The methylsuccinyl-CoA dehydrogenase (MCD)3 is a member of the flavin-dependent acyl-CoA dehydrogenase (ACD) family. MCD catalyzes the oxidation of the α-branched (2S)-methylsuccinyl-CoA into the corresponding trans-2-enoyl-CoA thioester, mesaconyl-CoA. The enzyme plays a crucial role in the ethylmalonyl-CoA pathway for acetyl-CoA assimilation in many α-proteobacteria (e.g. Rhodobacter sphaeroides, Methylobacterium extorquens, and Paracoccus denitrificans), actinobacteria (e.g. Streptomyces spp. and Frankia spp.), and possibly spirochaetes (e.g. Leptospira spp.). The α,β-desaturation of the CoA thioester is initiated by a proton abstraction from the α-carbon by a conserved catalytically active glutamate and a hydride transfer from the β-carbon to the N5 of the FAD cofactor.

Here we report the high resolution structure of MCD from P. denitrificans (PdMCD) that catalyzes the unprecedented α,β-desaturation of an α-methyl branched dicarboxylic acid CoA thioester. PdMCD forms a homodimer, consistent with our gel filtration analysis. The obtained well-ordered high-resolution electron density map allowed us to model almost the entire polypeptide chain (missing only 10 N-terminal residues) as well as the FAD cofactor in both active sites. Nevertheless, we also observed electron densities at the surfaces of each monomer that allowed the modeling of the adenosyl phosphate parts of CoA or its derivative. In contrast to canonical tetrameric ACDs, PdMCD possesses an additional ∼170-amino acid extension at the N terminus. However, when superimposing the PdMCD monomer with the MCAD tetramer, it becomes apparent that the N-terminal ∼170-residue extension of PdMCD structurally mimics the dimer–dimer interface of MCAD. By emulating the dimer–dimer interface found in the tetrameric ACDs, the N-terminal extension of PdMCD probably stabilizes the PdMCD dimer. The cofactor FAD binds to PdMCD in a “drawn-out” conformation, as observed for other ACDs. Both subunits of the MCD dimer contribute to the binding of FAD, which adopts a “butterfly-like” conformation in respect to the isoalloxazine ring. In PdMCD, however, helix E is shifted >2 Å to the back of the active site compared with IBD and MCAD, providing even more space, probably to accommodate the terminal carboxylic acid group of methylsuccinyl-CoA. The carboxylic acid group of the substrate could potentially interact with three arginine residues (Arg-252, Arg-376, and Arg-421) that are all in close proximity.

>MKDMPAMPADTPSALLALAGEALPELESLQSRATEALRALVAPAGKPQPALLEQHQHAAHALSWLTTYVESIRQLSGWAGRLAEAGNLGRIEALILQIGLGEYLGQIAGGIPMSQTEFARLSDLELDWQPGEAAAKLMRGNTAPARAELARLMQDNHGRATFGATGLDEDLEMIRDQFRRYAEERVIPNAHEWHLKDQLIPMEIIEELAELGVFGLTIPEEFGGLGLSKASMVVVTEELSRGYIGVGSLGTRSEIAAELILCGGTEAQKAKWLPGLASGEILSTAVFTEPNTGSDLGSLRTRAVRDGEDWVVTGNKTWITHAQRTHVMTLLARTDPETTDWRGLSMFLAEKEPGTDDDPFPTPGMTGGEIEVLGYRGMKEYELGFDGFRIKGENLLGGEPGRGFKQLMETFESARIQTAARAVGVAQSAAEIGMRYAVDRKQFGKSLIEFPRVADKLAMMAVEIMIARQLTYFSAWEKDHGRRCDLEAGMAKLLGARVAWAAADNALQIHGGNGFALEYAISRVLCDARILNIFEGAAEIQAQVIARRLLD[2x]> MSKPQNNDTLELDDILSQPVKDKERFAAFMMRKLAENKPAQNDNLFGNFKLDFDLDFEVPLIKKSQAKPKSKLPEVQPLGELVSKNSAATEKVNEPPVDQAPNENVPPRRSPTLSPNNRRSMRRSGNVPGSDKLRRHAIRRRSRSCGRQLLPEFEETVNLTRSISSPVNFLPEISSTPCTEKQKEEVAKNTTRVETDKPAEKPMELSQEPEPENPLQTKVTSPARNPILAAEIEQICKERQSSFHKNVLQLDYSGRAPYSRPPTPSSPSVAGLRRTYTMEKGPAPGQLLLSPSHRYDTPSKMPVVKAKRFNQELMVPDTPERQSHDPAWQSEPQPEFVVPETQPQDLGELVQTLSRSAISPIVVINTSNSNRSVRRDAVAMKSVPTSPVTALSSPPIAPSPRRSAAASPQKSIAQLPRVEENMDAIMTDDESDEHPSTVPLNLAPSGGNTTRQRRLRSSNRARATIESQESSMRLLNLHKSVNAKKSKPRKTAIPLNKAPSAPINGEQFARELTRMSNYEILDLRKRNSLNEIYPLNGHRNHRSEKLILEEEIQRELLRRNLMDEAEGLPKQQSSDDSNEDYIPVPPKTQSLRTKSNDRSQGRGRPRSTRRDLPMTTELVNYLGLSQTLETRRKSSKDGKRCLYTKGSSDHEDNDSLSPVKLPRLSKSIQIVPPPPVSLRYSQSLQNLPCSGKFDFDNVVMAAPPDFHDSVNSDAIEIAPPPPEYVVNTRGRSTSGRKSNKNDLVLPPPGYEGGQEEEHDERPSQPRCTAKELQQSTQNGRRAMENELVPPPIEYVEEENRNNEQSRRSTKNGNLVDRNTHNAVEYCEPPEPPEYDDSDHGQASILRRSGKKLQHSKQSVQKSNKEQIIAPSYENNEDYDSDEEPIYNEEYGKEESQNKNVTRRKSDKDEMASHTLECIEGPDPNWNSSCNKQNRNHQNASKSKENDKLANRSSKSQKLSNPRQNAVGTEKSVALSNRGEECTEKSSDVMESLRVNTPTPPIDQNSDDVPSRNPSPSRTLLSDDVPSTSRAALEFLQRSQNMSKSRPPDESSADVVFKKPLAPAPRAKSKKGKSEVDKLKLAKMPVEAEELNTTGIRRSKRGQVPLQMSWCHTMDPSKFNFMSGFIEPRSKNSKTKKGNLSKAKKASATKPKPTVEKNLPDNRGPLCSSTPRISEKLPGAIPHSESLGLSTLTWEETEVQAEAEKVPKKRGRPKKAVGGVQTDTEAEPEPEPEPMISSVAPLTSDQEEPDVPDEQAPYTEAALGPVVFSTPLRDEQEEASTKLMQWLRGVGDAPPSASMSDENASVSSANELIFYQVDGIDYAFYNTKEKAMLGYMRFKPYQKRSMKQAKVHPLKLLVQFGEFNVETLAVGEEKEVHSVLRVGDMIEIDRGTRYSIQNAIDKVSVLMCIRS

Centromeres are microtubule attachment sites on chromosomes defined by the enrichment of histone variant CENP‐A‐containing nucleosomes. To preserve centromere identity, CENP‐A must be escorted to centromeres by a CENP‐A‐specific chaperone for deposition. Instead, fly‐specific CAL1 appears to combine the roles of both HJURP and the Mis18 complex: pre‐nucleosomal CENP‐A recognition and its targeting to the centromere for deposition, respectively (Phansalkar et al, 2012). In this study, we present the structural basis for the recognition of CENP‐A/H4 and CENP‐C by CAL1.

Crystallisation trials carried out with CENP‐C1264–1411 alone and in complex with CAL1 produced diffraction quality crystals which diffracted X‐rays to about 1.8 and 2.3 Å, respectively. The twofold axis of the CENP‐C1264–1411 dimer was aligned with the crystallographic twofold axis. Consequently, just one molecule was present in the asymmetric unit. As expected, CENP‐C1264–1411 domain forms a cupin fold almost entirely made of β strands forming a β‐barrel with a helix preceding the cupin domain. The β strands assemble into two β sheets: a six‐stranded (β1‐β2‐β3‐β10‐β5‐β8) and a four‐stranded (β4‐β9‐β6‐β7). Dimerisation of CENP‐C cupin domain is mediated by a back‐to‐back arrangement of six‐stranded β‐sheets. In this arrangement, the loop connecting the N‐terminal α helix (α1) to β1 crosses over to its dimeric counterpart resulting in a “roof”‐like positioning of α‐helices on top of the β barrels. The surface area buried at the dimerisation interface is 1,706 Å2 which is about 50% of the total solvent accessible surface area. The interactions stabilising the dimerisation are predominantly hydrophobic involving residues L1283, W1286, L1287, L1312, L1314, Y1325, Y1335, M1407 and L1357. Structural comparison of dm and budding yeast CENP‐C cupin domains showed that although these domains share only weak similarity at the amino acid sequence level (21%), the overall fold conferring the β barrel structure is conserved.Chagas disease is caused by the protozoan parasite Trypanosoma cruzi, which is transmitted by blood-sucking reduviid bugs of the subfamily Triatominae. The cysteine protease cruzain is considered to be an attractive target for therapeutic intervention in the treatment of Chagas disease and the vinyl sulfone K777 (1) has been developed as an irreversible inhibitor of this enzyme. The human enzymes most closely related to cruzain are the cathepsins, in particular cathepsin L, and these have been targeted using the nitrile ‘warhead’ to form a covalent bond with the catalytic cysteine in a reversible manner.

Nitrile-based cysteine protease inhibitors targeted at rhodesain have also been shown to inhibit cruzain and a library of cathepsin inhibitors has been used as a source of antiparasitic leads. The design objectives of this study were to explore and map structure-activity relationships (SARs) for dipeptidyl nitrile inhibitors of cruzain and to evaluate compounds based on this scaffold for their trypanocidal activity. The dipeptidyl nitrile scaffold, as exemplified by 5, was adopted for this study since it is an established starting point for synthesis of Papain-like cysteine protease inhibitors and the P2 and P3 substituents can be varied easily using readily available synthetic building blocks.

>[5x]APAAVDWRARGAVTAVKDQGQCGSCWAFSAIGNVECQWFLAGHPLTNLSEQMLVSCDKTDSGCSGGLMNNAFEWIVQENNGAVYTEDSYPYASGEGISPPCTTSGHTVGATITGHVELPQDEAQIAAWLAVNGPVAVAVDASSWMTYTGGVMTSCVSEQLDHGVLLVGYNDSAAVPYWIIKNSWTTQWGEEGYIRIAKGSNQCLVKEEASSAVVG>SQIPASEQETLVRPKPLLLKLLKSVGAQK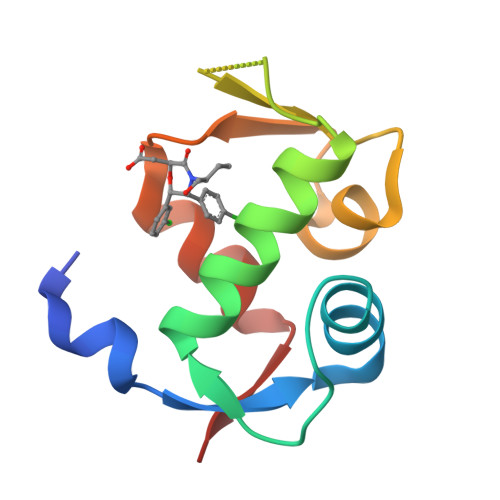DTYTMKEVLFYLGQYIMTKRLYDEKQQHIVYCSNDLLGDLFGVPSFSVKEHRKIYTMIYRNLVVVN[3x]>[2x]SNMNEKVLVLIVGTNPLPNYVVGSHLKEKYDKFVLIYSEKNDKINQNSTYDYAKKLKE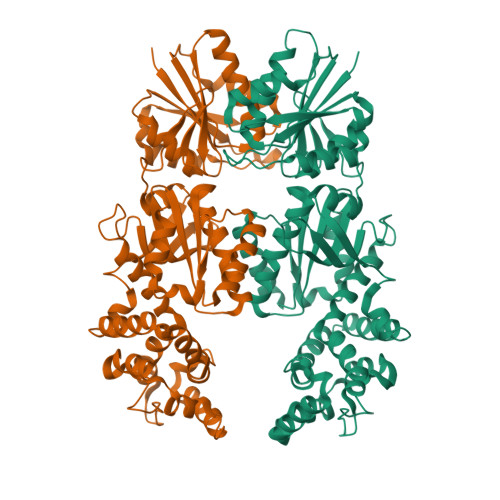HLNLNDKCIFLPLSDVSNSEKIINDLREKFPSEDFVEVHLNYTGGTKTMVVHIYNFLKEKFKNNKIKFEGSYLDARDYKLVYDYSEEAISLKDTIKIDINTLLSIHLYEDIHFEFYDTYSYKQKFVDSFDKISQEIEKAIKDDKGEDFVKWLEDPFRKIFKGENKLLEKTAKFKKHIEKLLKDNDSSPIVKFNEKTPQFIWDILNAFPEGKKLNDGQKLWIPDDKITNDNLSSRVKDTVEFLNGKWFEWYVYSQIKSELLDRKLKEGEHFGISLKAQKKDSPYFELDIFLINGYQLIGISLTTSSTRELCKLKGFEVIHRVRQIGGDESKAILITGMDKSKTEDLQKDLAYETGSTQKRFVVFGIDDWADIGSKICEEVFK> MRNGRTLLRWAGVLAATAIIGVGGFWSQGTTKALPEGPGEKRADLIEIGAMERFGKLDLPKVAFRHDQHTTAVTGMGKDCAACHKSKDGKMSLKFMRLDDNSAAELKEIYHANCIGCHTDLAKAGKKTGPQDGECRSCHNPKPSAASSWKEIGFDKSLHYRHVASKAIKPVGDPQKNCGACHHVYDEASKKLVWGKNKEDSCRACHGEKPVDKRPALDTAAHTACISCHMDVAKTKAETGPVNCAGCHAPEAQAKFKVVREVPRLDRGQPDAALILPVPGKDAPREMKGTMKPVAFDHKAHEAKANDCRTCHHVR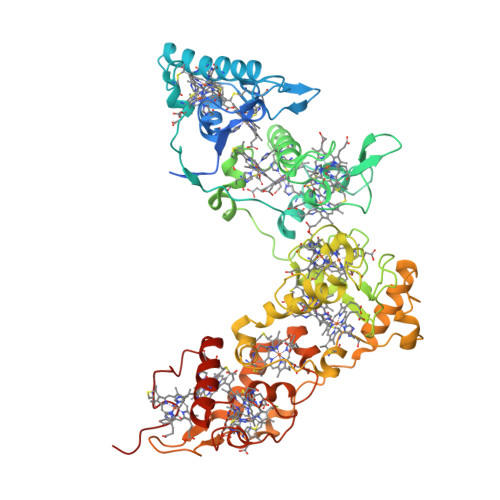IDTCTACHTVNGTADSKFVQLEKAMHQPDSMRSCVGCHNTRVQQPTCAGCHGFIKPTKSDAQCGVCHVAAPGFDAKQVEAGALLNLKAEQRSQVAASMLSARPQPKGTFDLNDIPEKVVIGSIAKEYQPSEFPHRKIVKTLIAGIGEDKLAATFHIEKGTLCQGCHHNSPASLTPPKCASCHGKPFDADRGDRPGLKAAYHQQCMGCHDRMKIEKPANTACVDCHKERAK> MTRRYLKYYIFVTLLFFVQVINNVLCAPDNKQEQGKYLNRTINILNAGKNIAKSYGHNKLKPIHILSALAKSDYGSTLFKENNVNAANLKEYIDIALEQTRAGAPLDNKSKIVNSAE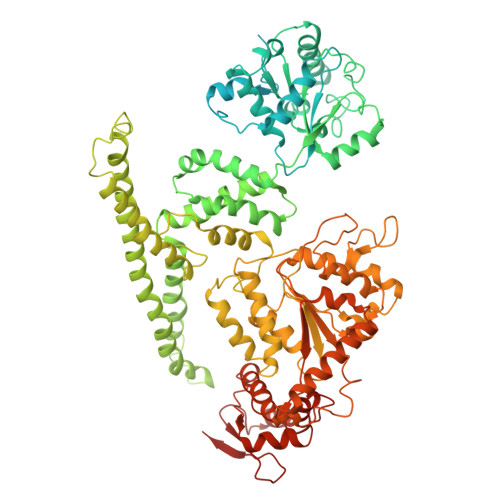VKETLALAEAAANKYKSPKVDVEHLLSGLSNDELVNEIFNEVYLTDEAIKAILKRKFEKTKKDKDGKTGTLYIEQFGSNMNEKVRNGKLQGIYGRDEEIRAIIESLLRYNKNSPVLVGNPGTGKTTIVEGLVYRIEKGDVPKELQGYTVISLNFRKFTSGTSYRGEFETRMKNIIKELKNKKNKIILFVDEIHLLLGAGKAEGGTDAANLLKPVLSKGEIKLIGATTIAEYRKFIESCSAFERRFEKILVEPPSVDMTVKILRSLKSKYENFYGINITDKALVAAAKISDRFIKDRYLPDKAIDLLNKACSFLQVQLSGKPRIIDVTERDIERLSYEISTLEKDVDKVSKKKYNKLIKEFEEKKEQLKKYYEEYVITGERLKRKKEIEKKLNDLKELTQNYVYSNKEPPIELQNSLKEAQQKYLELYKETVAYVEAKTHNAMNVDAVYQEHVSYIYLRDSGMPLGSLSFESSKGALKLYNSLSKSIIGNEDIIKSLSDAVVKAATGMKDPEKPIGTFLFLGPTGVGKTELAKTLAIELFNSKDNLIRVNMSEFTEAHSVSKITGSPPGYVGFSDSGQLTEAVREKPHSVVLFDELEKAHADVFKVLLQILGDGYINDNHRRNIDFSNTIIIMTSNLGAELFKKKLFFDADNSGTPEYKRVMEDVRLSLIKKCKKVFKPEFVNRIDKIGVFEPLNKKNLHKIVALRFKKLEKRLEEKNIQVSVSEKAIDYIIDQSYDPELGARPTLIFIESVIMTKFAIMYLKKELVDDMDVFVDYNSKAKNLVINLSKT> MSDAKVFGKCEFAELLKRDYYLSNDDIKNWVCIAEFESSFNTAAI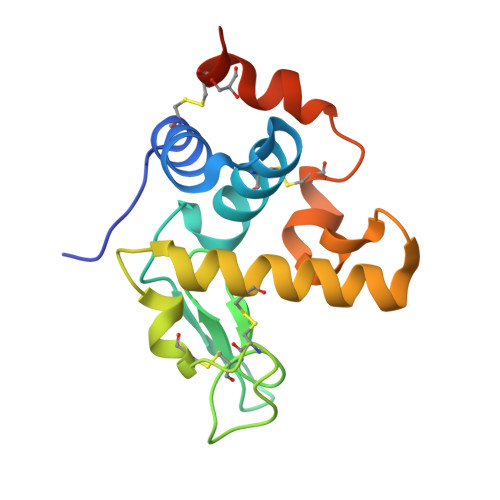NRNRNRSTDYGIFQINNKYWCGSDYGKNVCKIPCSDLMSDDITEALRCAETIRRDTERFRGRGKGYSAWVAYNSKCKNRDLDQYMAECWSHGSNSVFPF> GSHMDASVMSTTYALSAAQTEIWLAQQLYPDSPVYNIAQYTVIEGVIEPAVFEAALRQVIDEADTLRLQFIDSDDGLRQRIGTPAWSMPVLDLTAQADPQAAAQAWMRADYQQPVNLTQGPLFCYALLKVAPAQWMWYQRYHVIMMDGYGAYLIAQRVAYVYSALCEGTTPAECDFGSILQLLESDAQYQISAQRAQDEAYWLKHCANWSEPATLASRSAPVLQQRLRQTTYLAIQALGDTAPDARRLAQFMTAAMAAYLYRFTGEQDVVLGLPVKVRFGADRHIPGMKSNTLPLRLTMRPGMNLSSLMQ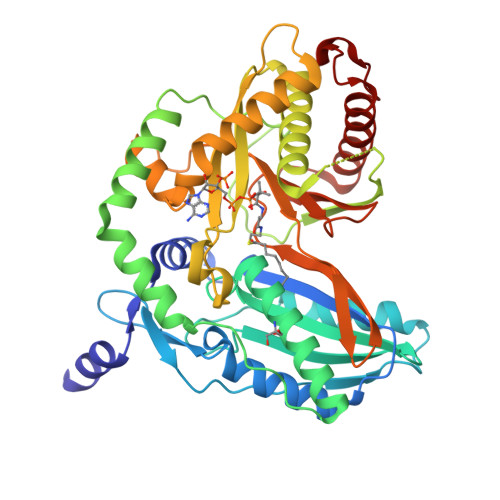QAAQEMQSGLRHQRYPSEALRRQLGMPSGQRLFGTTVNVMPFDLDLSFGGYSATNHNLLNGPAEDLMLGVYWTPGSHQLRIDFDANPACYTPEGLGAHQRRFIRFMQVLAADATQPIDSIDLLD>MAKLTIESMPLSVAEGKEVLLLVHNLPQHLFGYSWYKGERVDGNSQIVGYVIGTQQATPGAAYSGRETIYTN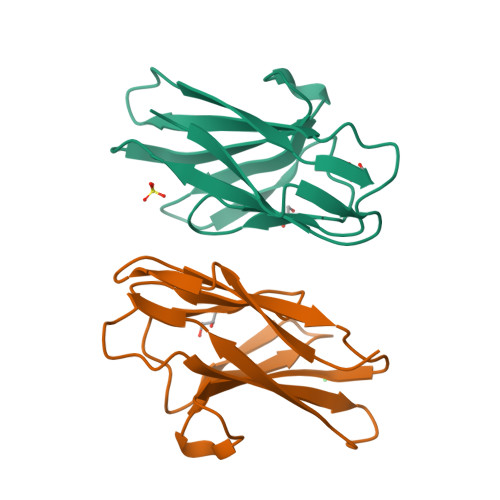ASLLIQNVTQNDIGFYTLQVIKSDLVNEEATGQFHVY[2x]> MSRNNDINAEVVSVSPNKLKISVDDLEEFKIAEEKLGVGSYLRVSDNQDVALLAIIDNFSIEVKESQKQKYMIEASPIGLVKNGKFYRGGDSLALPPKKVEPAKLDEIISIYSDSIDINDRFTFSSLSLNTKVSVPVNGNRFFNKHIAIVGSTGSGKSHTVAKILQKAVDEKQEGYKGLNNSHIIIFDIHSEYENAFPNSNVLNVDTLTLPYWLLNGDELEELFLDTEANDHNQRNVFRQAITLNKKIHFQGDPATKEIISFHSPYYFDINEVINYINNRNNERKNKDNEHIWSDEEGNFKFDNENAHRLFKENVTPDGSSAGALNGKLLNFVDRLQSKIFDKRLDFILGEGSKSVTFKETLETLISYGKDKSNITILDVSGVPFEVLSICVSLISRLIFEFGYHSKKIKRKSNENQDIPILIVYEEAHKYAPKSDLSKYRTSKEAIERIAKEGRKYGVTLLLASQR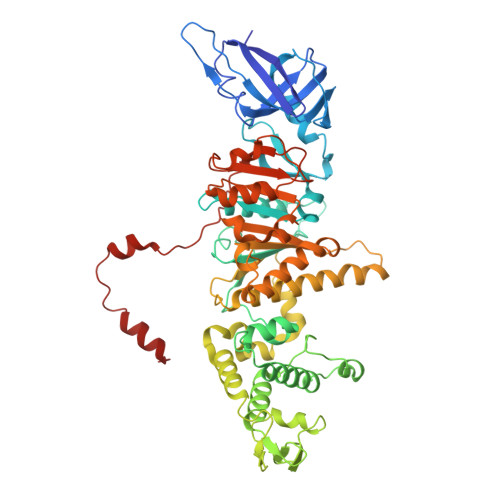PSEISETIFSQCNTFISMRLTNPDDQNYVKRLLPDTVGDITNLLPSLKEGEALIMGDSISIPSIVKIEKCTIPPSSIDIKYLDEWRKEWVDSEFDKIIEQWSKS>MIVMRVKVNEKQFDMIIDKLKLMVYEYNTKIKEYGVYLKPYHIVYKNSKRYIYIGKYWYKLEKIGGKLKWIYLGKTKPIQNMPNPPQIPESTIIKEDNEYIVDEKILYDLE[2x]

We identify a hitherto uncharacterized protein factor that we term UBP (ucm-binding protein) that interacts sequence-specifically with the ucm and determine the structure of the protein both in isolation and when bound to DNA. UBP is a highly abundant protein, and we reveal that it plays a role akin to bacterial nucleoid-associated proteins with over 300 binding sites on the Sulfolobus chromosome. Importantly, UBP interacts with the N-terminal domains of MCM. Taken together, our data provide evidence that UBP functions as a general nucleoid-associated protein that plays a key role in facilitating the egress of the MCM replicative helicase from DNA replication origins.

To gain further insight into the function of the UBP protein, we determined its structure using X-ray crystallography. The structure of the protein, solved to 2.74 Å resolution, revealed a homodimer. The overall conformation is saddle-shaped with a basic, concave undersurface and more acidic on the outer, convex surface. The concave surface is maximally 32 Å wide with the stirrups at the bottom of the saddle approximately 22 Å apart. Homodimerization is mediated by a reciprocal strand-swap of the C-terminal beta strands of the protomers. This strand interacts with the neighbor, forming a 5-strand beta sheet. The interprotomer interface encompasses 1662.4 Å2. Examination of the structure reveals a potential π-stacking interaction between tyrosine 100 at the base of the C-terminal beta-strand of one protomer and phenylalanine 13 of its partner. We mutated these residues to alanine and in both instances observed an altered profile on gel filtration chromatography in agreement with destabilization of the dimer and an elevated population of monomer species. Our initial determination of the homodimeric structure of UBP in the absence of DNA suggested the establishment of a symmetric structure of UBP at the origin.>GAGSTAGKVIKCKAAVLWEEKKPFSIEEVEVAPPKAHEVRIKMVATGICRTDDHVVSGTLVTPLPVIAGHEAAGIVESIGEGVTTVRPGDKVIPLFTPQCGKCRVCKHPEGNFCLKNDLSMPRGTMQDGTSRFTCRGKPIHHFLGTSTFSQYTVVDEISVAKIDAASPLEKVCLIGCGFSTGYGSAVKVAKVTQGSTCAVFGLGGVGLSVIMGCKAAGAARIIGVDINKDKFAKAKEVGATECVNPQDYKKPIQEVLTEMSNGGVDFSFEVIGRL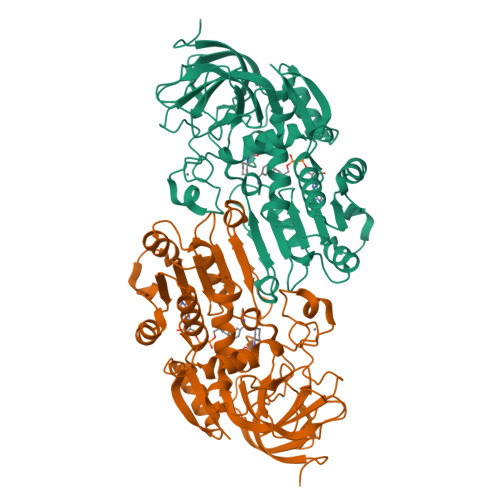DTMVTALSCCQEAYGVSVIVGVPPDSQNLSMNPMLLLSGRTWKGAIFGGFKSKDSVPKLVADFMAKKFALDPLITHVLPFEKINEGFDLLRSGESIRTILTF[2x]Here, we addressed the problem of accurate structural validation with cryo-EM-based methodologies for determining the structures of up to megadalton-scale DNA objects in solution, together with molecular-dynamics-based methods for building pseudoatomic models in a semiautomated fashion. The library of objects includes four brick-like multilayer DNA origami objects with increasing internal floppiness, a barrel-like 126-helix bundle, two variants of a multidomain object called Twisttower, a design variant v2 of a previously reported object called the Pointer, a small 16-helix bundle, four variants of a hinged-beam-like object, two variants of a dumbbell-like object, and five variants of a six-helix tube featuring asymmetric markers at either end as reporters for twist and one ten-helix tube. We constructed pseudoatomic models for six different objects. The fitting was validated using Fourier shell correlation against the cryo-EM half-maps and the models show good cross-correlation with the cryo-EM maps.

The Twisttower design allowed us to systematically study twist deformations, and how they may be removed, in a square-lattice packing context as a function of cross-sectional area. To remove the global twist deformation, the internal design specifics must be changed such that the right-handed internal torques are mechanically balanced by counteracting left-handed torques. This may be achieved by locally deviating from the default eight-base-pair crossover spacing design rules following previously discussed concepts, by reducing the average bases between crossovers to achieve the native 10.5 base pairs per turn. We thus designed and solved a cryo-EM structure of a refined variant of the Twisttower in which we eliminated the global twist deformations. As a result, we obtained a more orderly object with a more regular square-lattice structure (right). We applied this analysis also to the twist-corrected variant of the Twisttower and the hinged-beam-like object v4.

> AAAAGAAGCCACCCTCCCGTCACCGACTTGAG;> TCATAAATCAGTTCAGAAAACGAGTCTAGCTGTGCCTGAGTACAAAAT;> ATTCATTGAATCCCCAAGAATAACTTAATTAAATAAGGAGAAACCA;> CATTACCGAGGGGGTAATAGTACACTATCA;> AAAATCAGAAATCACCTCAAATCACCATCAATGTCTGGAGTTTTT;> TTTTTTAAATTTAAAGAAGATGATGATTTTTTAACAAACATCAAG;> AGCCAGCATGAGGGAGGATAAAAATTTTTAGATAATCGTACAAACAAG;> TTCTGACCAATATATTTTAATGGAAACAGTTTTTTTACATAAATCAAT;> CCAGAGCCGCCATCTTGGCATTTTCGGTCTTTTTTTTTTATAGCCCCCTTATCCATCGAT;> TTAGTTAAAAGACAAACCGCGCCCAATAGCATCGTAGG;> TGATAGACGGTTTTTCGCCCTTTGACGTTGGAGTCCACGTTCTTTAATAGTGGACTCTTGTTCCAAACTGGAACAACACTCAACCCTATCTCGGGCTATTCTTTTGATTTATAAGGGATTTTGCCGATTTCGGAACCACCATCAAACAGGATTTTCGCCTGCTGGGGCAAACCAGCGTGGACCGCTTGCTGCAACTCTCTCAGGGCCAGGCGGTGAAGGGCAATCAGCTGTTGCCCGTCTCACTGGTGAAAAGAAAAACCACCCTGGCGCCCAATACGCAAACCGCCTCTCCCCGCGCGTTGGCCGATTCATTAATGCAGCTGGCACGACAGGTTTCCCGACTGGAAAGCGGGCAGTGAGCGCAACGCAATTAATGTGAGTTAGCTCACTCATTAGGCACCCCAGGCTTTACACTTTATGCTTCCGGCTCGTATGTTGTGTGGAATTGTGAGCGGATAACAATTTCACACAGGAAACAGCTATGACCATGATTACGAATTCGAGCTCGGTACCCGGGGATCCTCAACTGTGAGGAGGCTCACGGACGCGAAGAACAGGCACGCGTGCTGGCAGAAACCCCCGGTATGACCGTGAAAACGGCCCGCCGCATTCTGGCCGCAGCACCACAGAGTGCACAGGCGCGCAGTGACACTGCGCTGGATCGTCTGATGCAGGGGGCACCGGCACCGCTGGCTGCAGGTAACCCGGCATCTGATGCCGTTAACGATTTGCTGAACACACCAGTGTAAGGGATGTTTATGACGAGCAAAGAAACCTTTACCCATTACCAGCCGCAGGGCAACAGTGACCCGGCTCATACCGCAACCGCGCCCGGCGGATTGAGTGCGAAAGCGCCTGCAATGACCCCGCTGATGCTGGACACCTCCAGCCGTAAGCTGGTTGCGTGGGATGGCACCACCGACGGTGCTGCCGTTGGCATTCTTGCGGTTGCTGCTGACCAGACCAGCACCACGCTGACGTTCTACAAGTCCGGCACGTTCCGTTATGAGGATGTGCTCTGGCCGGAGGCTGCCAGCGACGAGACGAAAAAACGGACCGCGTTTGCCGGAACGGCAATCAGCATCGTTTAACTTTACCCTTCATCACTAAAGGCCGCCTGTGCGGCTTTTTTTACGGGATTTTTTTATGTCGATGTACACAACCGCCCAACTGCTGGCGGCAAATGAGCAGAAATTTAAGTTTGATCCGCTGTTTCTGCGTCTCTTTTTCCGTGAGAGCTATCCCTTCACCACGGAGAAAGTCTATCTCTCACAAATTCCGGGACTGGTAAACATGGCGCTGTACGTTTCGCCGATTGTTTCCGGTGAGGTTATCCGTTCCCGTGGCGGCTCCACCTCTGAAAGCTTGGCACTGGCCGTCGTTTTACAACGTCGTGACTGGGAAAACCCTGGCGTTACCCAACTTAATCGCCTTGCAGCACATCCCCCTTTCGCCAGCTGGCGTAATAGCGAAGAGGCCCGCACCGATCGCCCTTCCCAACAGTTGCGCAGCCTGAATGGCGAATGGCGCTTTGCCTGGTTTCCGGCACCAGAAGCGGTGCCGGAAAGCTGGCTGGAGTGCGATCTTCCTGAGGCCGATACTGTCGTCGTCCCCTCAAACTGGCAGATGCACGGTTACGATGCGCCCATCTACACCAACGTGACCTATCCCATTACGGTCAATCCGCCGTTTGTTCCCACGGAGAATCCGACGGGTTGTTACTCGCTCACATTTAATGTTGATGAAAGCTGGCTACAGGAAGGCCAGACGCGAATTATTTTTGATGGCGTTCCTATTGGTTAAAAAATGAGCTGATTTAACAAAAATTTAATGCGAATTTTAACAAAATATTAACGTTTACAATTTAAATATTTGCTTATACAATCTTCCTGTTTTTGGGGCTTTTCTGATTATCAACCGGGGTACATATGATTGACATGCTAGTTTTACGATTACCGTTCATCGATTCTCTTGTTTGCTCCAGACTCTCAGGCAATGACCTGATAGCCTTTGTAGATCTCTCAAAAATAGCTACCCTCTCCGGCATTAATTTATCAGCTAGAACGGTTGAATATCATATTGATGGTGATTTGACTGTCTCCGGCCTTTCTCACCCTTTTGAATCTTTACCTACACATTACTCAGGCATTGCATTTAAAATATATGAGGGTTCTAAAAATTTTTATCCTTGCGTTGAAATAAAGGCTTCTCCCGCAAAAGTATTACAGGGTCATAATGTTTTTGGTACAACCGATTTAGCTTTATGCTCTGAGGCTTTATTGCTTAATTTTGCTAATTCTTTGCCTTGCCTGTATGATTTATTGGATGTTAATGCTACTACTATTAGTAGAATTGATGCCACCTTTTCAGCTCGCGCCCCAAATGAAAATATAGCTAAACAGGTTATTGACCATTTGCGAAATGTATCTAATGGTCAAACTAAATCTACTCGTTCGCAGAATTGGGAATCAACTGTTATATGGAATGAAACTTCCAGACACCGTACTTTAGTTGCATATTTAAAACATGTTGAGCTACAGCATTATATTCAGCAATTAAGCTCTAAGCCATCCGCAAAAATGACCTCTTATCAAAAGGAGCAATTAAAGGTACTCTCTAATCCTGACCTGTTGGAGTTTGCTTCCGGTCTGGTTCGCTTTGAAGCTCGAATTAAAACGCGATATTTGAAGTCTTTCGGGCTTCCTCTTAATCTTTTTGATGCAATCCGCTTTGCTTCTGACTATAATAGTCAGGGTAAAGACCTGATTTTTGATTTATGGTCATTCTCGTTTTCTGAACTGTTTAAAGCATTTGAGGGGGATTCAATGAATATTTATGACGATTCCGCAGTATTGGACGCTATCCAGTCTAAACATTTTACTATTACCCCCTCTGGCAAAACTTCTTTTGCAAAAGCCTCTCGCTATTTTGGTTTTTATCGTCGTCTGGTAAACGAGGGTTATGATAGTGTTGCTCTTACTATGCCTCGTAATTCCTTTTGGCGTTATGTATCTGCATTAGTTGAATGTGGTATTCCTAAATCTCAACTGATGAATCTTTCTACCTGTAATAATGTTGTTCCGTTAGTTCGTTTTATTAACGTAGATTTTTCTTCCCAACGTCCTGACTGGTATAATGAGCCAGTTCTTAAAATCGCATAAGGTAATTCACAATGATTAAAGTTGAAATTAAACCATCTCAAGCCCAATTTACTACTCGTTCTGGTGTTTCTCGTCAGGGCAAGCCTTATTCACTGAATGAGCAGCTTTGTTACGTTGATTTGGGTAATGAATATCCGGTTCTTGTCAAGATTACTCTTGATGAAGGTCAGCCAGCCTATGCGCCTGGTCTGTACACCGTTCATCTGTCCTCTTTCAAAGTTGGTCAGTTCGGTTCCCTTATGATTGACCGTCTGCGCCTCGTTCCGGCTAAGTAACATGGAGCAGGTCGCGGATTTCGACACAATTTATCAGGCGATGATACAAATCTCCGTTGTACTTTGTTTCGCGCTTGGTATAATCGCTGGGGGTCAAAGATGAGTGTTTTAGTGTATTCTTTTGCCTCTTTCGTTTTAGGTTGGTGCCTTCGTAGTGGCATTACGTATTTTACCCGTTTAATGGAAACTTCCTCATGAAAAAGTCTTTAGTCCTCAAAGCCTCTGTAGCCGTTGCTACCCTCGTTCCGATGCTGTCTTTCGCTGCTGAGGGTGACGATCCCGCAAAAGCGGCCTTTAACTCCCTGCAAGCCTCAGCGACCGAATATATCGGTTATGCGTGGGCGATGGTTGTTGTCATTGTCGGCGCAACTATCGGTATCAAGCTGTTTAAGAAATTCACCTCGAAAGCAAGCTGATAAACCGATACAATTAAAGGCTCCTTTTGGAGCCTTTTTTTTGGAGATTTTCAACGTGAAAAAATTATTATTCGCAATTCCTTTAGTTGTTCCTTTCTATTCTCACTCCGCTGAAACTGTTGAAAGTTGTTTAGCAAAATCCCATACAGAAAATTCATTTACTAACGTCTGGAAAGACGACAAAACTTTAGATCGTTACGCTAACTATGAGGGCTGTCTGTGGAATGCTACAGGCGTTGTAGTTTGTACTGGTGACGAAACTCAGTGTTACGGTACATGGGTTCCTATTGGGCTTGCTATCCCTGAAAATGAGGGTGGTGGCTCTGAGGGTGGCGGTTCTGAGGGTGGCGGTTCTGAGGGTGGCGGTACTAAACCTCCTGAGTACGGTGATACACCTATTCCGGGCTATACTTATATCAACCCTCTCGACGGCACTTATCCGCCTGGTACTGAGCAAAACCCCGCTAATCCTAATCCTTCTCTTGAGGAGTCTCAGCCTCTTAATACTTTCATGTTTCAGAATAATAGGTTCCGAAATAGGCAGGGGGCATTAACTGTTTATACGGGCACTGTTACTCAAGGCACTGACCCCGTTAAAACTTATTACCAGTACACTCCTGTATCATCAAAAGCCATGTATGACGCTTACTGGAACGGTAAATTCAGAGACTGCGCTTTCCATTCTGGCTTTAATGAGGATTTATTTGTTTGTGAATATCAAGGCCAATCGTCTGACCTGCCTCAACCTCCTGTCAATGCTGGCGGCGGCTCTGGTGGTGGTTCTGGTGGCGGCTCTGAGGGTGGTGGCTCTGAGGGTGGCGGTTCTGAGGGTGGCGGCTCTGAGGGAGGCGGTTCCGGTGGTGGCTCTGGTTCCGGTGATTTTGATTATGAAAAGATGGCAAACGCTAATAAGGGGGCTATGACCGAAAATGCCGATGAAAACGCGCTACAGTCTGACGCTAAAGGCAAACTTGATTCTGTCGCTACTGATTACGGTGCTGCTATCGATGGTTTCATTGGTGACGTTTCCGGCCTTGCTAATGGTAATGGTGCTACTGGTGATTTTGCTGGCTCTAATTCCCAAATGGCTCAAGTCGGTGACGGTGATAATTCACCTTTAATGAATAATTTCCGTCAATATTTACCTTCCCTCCCTCAATCGGTTGAATGTCGCCCTTTTGTCTTTGGCGCTGGTAAACCATATGAATTTTCTATTGATTGTGACAAAATAAACTTATTCCGTGGTGTCTTTGCGTTTCTTTTATATGTTGCCACCTTTATGTATGTATTTTCTACGTTTGCTAACATACTGCGTAATAAGGAGTCTTAATCATGCCAGTTCTTTTGGGTATTCCGTTATTATTGCGTTTCCTCGGTTTCCTTCTGGTAACTTTGTTCGGCTATCTGCTTACTTTTCTTAAAAAGGGCTTCGGTAAGATAGCTATTGCTATTTCATTGTTTCTTGCTCTTATTATTGGGCTTAACTCAATTCTTGTGGGTTATCTCTCTGATATTAGCGCTCAATTACCCTCTGACTTTGTTCAGGGTGTTCAGTTAATTCTCCCGTCTAATGCGCTTCCCTGTTTTTATGTTATTCTCTCTGTAAAGGCTGCTATTTTCATTTTTGACGTTAAACAAAAAATCGTTTCTTATTTGGATTGGGATAAATAATATGGCTGTTTATTTTGTAACTGGCAAATTAGGCTCTGGAAAGACGCTCGTTAGCGTTGGTAAGATTCAGGATAAAATTGTAGCTGGGTGCAAAATAGCAACTAATCTTGATTTAAGGCTTCAAAACCTCCCGCAAGTCGGGAGGTTCGCTAAAACGCCTCGCGTTCTTAGAATACCGGATAAGCCTTCTATATCTGATTTGCTTGCTATTGGGCGCGGTAATGATTCCTACGATGAAAATAAAAACGGCTTGCTTGTTCTCGATGAGTGCGGTACTTGGTTTAATACCCGTTCTTGGAATGATAAGGAAAGACAGCCGATTATTGATTGGTTTCTACATGCTCGTAAATTAGGATGGGATATTATTTTTCTTGTTCAGGACTTATCTATTGTTGATAAACAGGCGCGTTCTGCATTAGCTGAACATGTTGTTTATTGTCGTCGTCTGGACAGAATTACTTTACCTTTTGTCGGTACTTTATATTCTCTTATTACTGGCTCGAAAATGCCTCTGCCTAAATTACATGTTGGCGTTGTTAAATATGGCGATTCTCAATTAAGCCCTACTGTTGAGCGTTGGCTTTATACTGGTAAGAATTTGTATAACGCATATGATACTAAACAGGCTTTTTCTAGTAATTATGATTCCGGTGTTTATTCTTATTTAACGCCTTATTTATCACACGGTCGGTATTTCAAACCATTAAATTTAGGTCAGAAGATGAAATTAACTAAAATATATTTGAAAAAGTTTTCTCGCGTTCTTTGTCTTGCGATTGGATTTGCATCAGCATTTACATATAGTTATATAACCCAACCTAAGCCGGAGGTTAAAAAGGTAGTCTCTCAGACCTATGATTTTGATAAATTCACTATTGACTCTTCTCAGCGTCTTAATCTAAGCTATCGCTATGTTTTCAAGGATTCTAAGGGAAAATTAATTAATAGCGACGATTTACAGAAGCAAGGTTATTCACTCACATATATTGATTTATGTACTGTTTCCATTAAAAAAGGTAATTCAAATGAAATTGTTAAATGTAATTAATTTTGTTTTCTTGATGTTTGTTTCATCATCTTCTTTTGCTCAGGTAATTGAAATGAATAATTCGCCTCTGCGCGATTTTGTAACTTGGTATTCAAAGCAATCAGGCGAATCCGTTATTGTTTCTCCCGATGTAAAAGGTACTGTTACTGTATATTCATCTGACGTTAAACCTGAAAATCTACGCAATTTCTTTATTTCTGTTTTACGTGCAAATAATTTTGATATGGTAGGTTCTAACCCTTCCATTATTCAGAAGTATAATCCAAACAATCAGGATTATATTGATGAATTGCCATCATCTGATAATCAGGAATATGATGATAATTCCGCTCCTTCTGGTGGTTTCTTTGTTCCGCAAAATGATAATGTTACTCAAACTTTTAAAATTAATAACGTTCGGGCAAAGGATTTAATACGAGTTGTCGAATTGTTTGTAAAGTCTAATACTTCTAAATCCTCAAATGTATTATCTATTGACGGCTCTAATCTATTAGTTGTTAGTGCTCCTAAAGATATTTTAGATAACCTTCCTCAATTCCTTTCAACTGTTGATTTGCCAACTGACCAGATATTGATTGAGGGTTTGATATTTGAGGTTCAGCAAGGTGATGCTTTAGATTTTTCATTTGCTGCTGGCTCTCAGCGTGGCACTGTTGCAGGCGGTGTTAATACTGACCGCCTCACCTCTGTTTTATCTTCTGCTGGTGGTTCGTTCGGTATTTTTAATGGCGATGTTTTAGGGCTATCAGTTCGCGCATTAAAGACTAATAGCCATTCAAAAATATTGTCTGTGCCACGTATTCTTACGCTTTCAGGTCAGAAGGGTTCTATCTCTGTTGGCCAGAATGTCCCTTTTATTACTGGTCGTGTGACTGGTGAATCTGCCAATGTAAATAATCCATTTCAGACGATTGAGCGTCAAAATGTAGGTATTTCCATGAGCGTTTTTCCTGTTGCAATGGCTGGCGGTAATATTGTTCTGGATATTACCAGCAAGGCCGATAGTTTGAGTTCTTCTACTCAGGCAAGTGATGTTATTACTAATCAAAGAAGTATTGCTACAACGGTTAATTTGCGTGATGGACAGACTCTTTTACTCGGTGGCCTCACTGATTATAAAAACACTTCTCAGGATTCTGGCGTACCGTTCCTGTCTAAAATCCCTTTAATCGGCCTCCTGTTTAGCTCCCGCTCTGATTCTAACGAGGAAAGCACGTTATACGTGCTCGTCAAAGCAACCATAGTACGCGCCCTGTAGCGGCGCATTAAGCGCGGCGGGTGTGGTGGTTACGCGCAGCGTGACCGCTACACTTGCCAGCGCCCTAGCGCCCGCTCCTTTCGCTTTCTTCCCTTCCTTTCTCGCCACGTTCGCCGGCTTTCCCCGTCAAGCTCTAAATCGGGGGCTCCCTTTAGGGTTCCGATTTAGTGCTTTACGGCACCTCGACCCCAAAAAACTTGATTTGGGTGATGGTTCACGTAGTGGGCCATCGCCC;> AACGGAGATTTGTATTAGGAATACAAAAGGATCAGGACGATGCCACT;> TTTTTGCGCGAAACACTAAAACCAGCGATAAGAGGCAGAGGACTAAAGACTTT;> TTGAGATTTTGTGAATTATACCAGAACGTAACCAGCATCGGAACGAGG;> CTGACCTTCATCGCCTCCATGTTAATTACGAGCGTTTACCAGACGACG;> GTAATCTTGACAAGATTGAAAGACTCCAAAACTAAAGGATTTTCACGGCTGAGGC;> TTTTGTTTTGTCCAGACAGCCCTCATTTTTTTTTTTAGTTAGCGTAAC;> AGACGTTAGTAAATGAATTGTATTCTTAAAC;> CGGTTTATCAGCTTGTTGAAAATTTTTT;> GTTTCAGCAGCTTGATCATCGCCCACGCATAAGCATGATTAACAGTTA;> GGAGTGAGTTGCGGGATCGTCACCCCCGTATA;> GTGAATAAGGCTTTTTTTTTTTTGCCCTGACGAGAAAACCCATGTCAGGGAT;> TCATTCATGGTTTAATTTCAACTTTAATCAAATTTTCT;> AAAGCTGCTTCAACAGTATGGGATTTTGCTGATCTAAAGCTTGAGA;> ACCGGATAGGAACAAAAAAGGCTCCAAAAGGAGCCTTTCATCAAGA;> GGTCAATCGACCAACTGAGGCTTTTTGCAGGGTTCGGAACCTATTATT;> TACGTTAATAAAATTTTTTTTTTCGAACTAACGGAACCTCATTTTTTT;> TTGGGAAGGGCTCATTACCTTATGCGATTTACACCAGATTACAGGT;> CAAAATAGCAGATACATAACGCCCACATTCAACTAATCAACATTATTTTT;> AAAAGCCTACCAGTATAAAGCCATATCATTCTGCAGAACGCTGAGAC;> TTACTAGACGGAATCGCCAACATGCAGAAGCAAAGCGGAT;> TTTTTCGTTAAATATGGTTTGAAATATTTTTTCCGACCGTGTGAT;> ACGAAGGCGTACCGACTTTTGCCAATTAGCAAGGCCGGAACCGTAATC;> AAAACGAAATCCGCGCGCAGACAGGCGCATAGGCTGG;> AAATTCTTGTTTAGTATCATATGAAAGAATAAAATGTTTAGCCAGTA;> CCATTAAATAGTACCGGTGCCGTCTTACCAGCGCCAAAGA;> TTCATGAGAACGAGGACCTGCTGATAAATTGTGTCGATATACCAATACAGACC;> GGTATTAAACCAAGTCGTTATACCATTTTCGAGACTGGA;> TCGGCTGTCTTTCCTACGCTCAATAACAACG;> CAGTACAACAATAGGTAAGAACTAAAAATCAGAAAGATTCATCAG;> CGCCTGTATTCGTCACAGTATAGCCCGGATTTTTTTTTTATAGGTGTATCAC;> GCCGCTTAATAGAAATTCATTACCCAAATCCTTAGCCGGGAAGTTT;> AGTTAAAGTTCGGTCCTTTCGAGGTGAATT;> CCAGCTACAGCGTCTTTCCAGAGTAGACGGGGAACAAAG;> TTTTGCATTCCAGGTAATAAGTTTTTTTTTTTTTTAACGGGGTCAGTG;> AAGACTCCAATACATACATAAAGGTGGAAAGCATAAATCC;> GAGGAAACGCTAACGAATTTTATCCTGAATACCGCACT;> TATCCCAACAGATATAGAGTACCTTTAATTGCTGTACCAACATTAACAGAACCTAC;> TATTATTGCCAGTTACAAGATTAGTTGCTATTATTTTC;> AACAGTGCTCAGCAGCAACAACACCGATAGTTGCGCCGTCTTTCC;> GAAGGCTTATCCGGTCCTTAAATCAAAATAGAACCTCCGAGAGAAT;> ATTCTAAGAACGCTTTTTTGAGGCGTTTTAGCATATAACTTAACCTCC;> GCGGATAAAAAAGGTAACGGAAATTATTCATT;> TTAGGATTCAATAAACGTTTTAATGTCTTTACGATTCAAAAGGGTGAG;> AAGCAAATGCGCCTGTAAGAGGAAGCCCGAAAAAATGCAAAAACATTA;> CAGCTAACAAGAACGACAAGCAAGCCGTTTTTTTGCACATTAAGAGTTACCAGA;> TTATCAACAATAGATATCAATAAAATCATTCCATCCTATTTTGAAG;> AAGTCCTGAACAATTTTTTGAAAAATAATATCAGAACGCGATGCAAAT;> AGAACCGCCACCCTTTTTTTTTTTCAGAGCCACCACTAGCGTTTTTTT;> ATATAAAACCAACCTTAACCCTGCATAGTAAGAGCAACAAAGTAC;> ATAAGAGACTGTCCAGACGACGAAGCGGGGT;> CCATATTCAGTAGGGACACCGGAATCATAA;> CAGGAAGAACAATAATTTGAATTACCTTTT;> ATGAATATTAGATTTTGTTATTAATTTTATTTTTTTTTTAAAGTTTGAGTAA;> GTAAACGTAGGGTTATCCAATAAATCATAC;> CCAATAGGTGTTAAATTCGGCCTCACCGCTTCCAGCAACCGCAAGAATTGGGTAAA;> ACTTCTGACATCTGCCCCGTCGGAAAGGGAAGAAAGCGAAAGCGGTCA;> TGGATTATCATATCAAAATTATTTTTGTATA;> GATTGTTGAGTCAATAGTGAATGGCTTAGGGACCATTGTTAAGCC;> TTTTTAACGCCATAACGGCGGATTGACCGCGGGGAAA;> AACTGTTGGGAAGTTTTTTTTTTGGCGATCGGTGCGTCGTCTCGTCCGGCAA;> GGCCTCTTCGCTATTCTTTGAATGATAATCTGACCCTG;> CAACCGATAAGACACCATAAAGCCTCAGAGCATTGTTAAACATATGTA;> CGGAAGCAAACTCCAACAGGTCAGAAAGATT;> GATACAGGGGAGGTTGCCTCAGAGCCGCCTTTTTTTTTTACCAGAACCACCAACCGGAAC;> GAAAATTCCGTAGAATTATTACGCAGTATGGACAATGAACTACAAAAACAACT;> TTTGTCACAATCAATAACAAACAAGCAGTCTC;> ACGGAATATATAAAATACCCAAAAGAACTGCCGATATA;> GTCATTTTTCGAGCTTTTTGCGGGAGAAGCCTTTATTTCATTAAGCA;> TTTTTAGTGTACTAGTAAGCGTCATATTTTTTTTTTCATGGCTTTTGATTTGGCCTT;> TGGCAACAAGTTTATATGCCCCCGTACCAGGTAGCAACGGCTACA;> GCTTAGAGCTTAATTAGGAAACCGATAGCCAGAATTAATGAGCGC;> GCTGAATACAACTAAAAGTAGTAGTAACCTGTTCTGGCCTTCCTGTAG;> TGAATTTACCGTTCCTTAGCAAACAGACGACCTTGAGTTGATATA;> ATTAAGACTCTGTAAAAGCAAATATTTAAATTGGCAAAGCAGTTTGAG;> ATAGCGATAGCTTAGTAGCTCAAGATTAGA;> TCATTAAAGCCGCCACAAAAGGGCGACATTTTTGCTCATGCCTAT;> TAAAGCTATAATACTCAAAGCGAACCAGACTCCTCAAGTGAAAGT;> AATCGGTTCCTTTTGATAAGAGCTGAAACAAGAAGGACATCGAGA;> TCGTCGCTATTAATTCCAATCGCTTGGGTTAACAGCCA;> AATTTTCCCTTAGTTTTTTAATCCTTGAAAACAAACAGAATCATCAAT;> CCACCACAGGCAGGTCAAAATCCGTACTCAGGAGGTTCGGGTAAACGAAAGA;> CCCTCAGAAACCGCCTCCCTCAGAAGTTTGCCCATTTGG;> ACCTTGCTCAATTTCACGGATTCGCCTGATTG;> ACCACCGGACCGCCACCCTCAGAGGATATTC;> ACCCTCATAGGTAAACCTGACTATAAATCATAGCGTCCAATACTG;> TTTCATCTTCATAATAATGAAAGCGAGAGGCTTTTGCATAAAAACATACGTA;> TCAGACTGTAGCGCGTCAGAGCCAAAGGTGAATATGGTGAGAGGGT;> CTTTAGCGAGTAGCGACAGAATCAGAGACAGAGTAGCACGAATTAG;> AAAGGCCGACGCAAGGGAAGGTAAATATTGAAGTAATT;> TAATGTGTATATTTTGACTTCAAATATCGCAACATGTTGCAGAGG;> ACATTTAAATAAATTATCTACAAAGGCTATCATAAAACGATGGCGAAA;> AGCAGCAACGTCACCATTATCAAGAACCGCCACCCTCAGCAAGCC;> ATGATATTCAACCGTAATGACCATTATAGTTAATTTAG;> ATGCCGGAGAGGGTACTCAAATGTTTCATCGAGAATCG;> CCCTGAACCTTACCAACGCAATAATAACGGAAGAAACGCA;> TTTTTAAAGTCAGATCTTACCGAAGCTTTTTTTTTTCCTTTTTAAGAAA;> TAATATCAGAGAGATAAAGAGCAATCCAAATATAAATATGTAATGCTG;> GAAATAGCAATAGCTAGGGTAATCTGAACA;> GAAACAATTCTGCGAACGAGTAGAATGGTCAAGCTGAGAA;> CAATAATACCCACAAAACAGGGAAGCGCATCCTAATTT;> AGAAACGATTTTTTGAACATAAAGAATTGACCTTTACATTTTT;> TTTAACGTCAAAATTTTTTATGAAAATAGCAGTACCTTTTTTTTT;> GTTTCATTTGCGGATGAGGCAAGGCAAAGAATTAGCAAAAGCCAGAA;> TTTTCCATATAATTTGGGGCGCGAGTTTTTTTTTTCTGAAAAGGTGGC;> TTAGCTATATTTTCACAGTTGATTCTGGAAAGTAAGCA;> AGATACATTTCGCAATTTAGTTTCATGTTT;> TTATCAAAATCATTTTTTTAGGTCTGAGAGACATGGCAATTTTTT;> TTTTTCTGAGCAAGAATTGAGGAAGGTTTTTTTTTTTTATCTAAAATAT;> CGCGCAGACAACTAATCGGCCAGTGAACGGATAACCTCAC;> ATTCATTAAAACAAAATTAATTTGCATCAACTTTAAA;> TCAATTACTTTTACATTACATTTGAGGATTTTTTTTTTTTTAGAAGTATTAG;> CGGGAGAAACGTCAGATATGTGAGTGAATA;> AGAAAAGCCCCAAAAACGACAACTAGATTAGATTTTGAAT;> CCTTCTGACTTGCTGGATTAGTAATAACATTTTTTTTTTTCACTTGCCTGAGTTTTTATA;> ACTTTCTCCGGCCTTTAGTGATGAAGGGTAAACTTAAATGAGACGCA;> AATTTGTGAGAGATAGCGGAAAAATTCTGCTC;> ATCGGCGCCAGTCACGACGTTGGGTCATTGACCAAGT;> TTTTTGTTGAAAGCTCAATCAATATCTTTTTTTTTTTGGTCAGTTGGCATACCGAAC;> TTTTTAAAAAAGCTTGGGCGGATAAAAAAAAGGGATAGCTCTCA;> ACTGATAGGGCTATTAATTCACCAGGAAAAACGCTCATGGCCATCAC;> CCCTAAAACAGCAGAATGCTGAACCTCAAATATCAAACCGTGGAGCC;> CATCGCCAGCCACGGGCCAAGCTTTCAGAGGCTATTTT;> TTAAAAACTTTAGGAGCACTAAGGCGAATTTGAGAGA;> ACGCCAGCGCCATTCGCACATCCTCATAACGG;> AGGCGATTGGGTTTTCAAACGTACAGCGCCAT;> GGGGGATGTGCTGCAAGAATCGACCTGAGA;> CAACAGCTCGTGCCAGCTGCTTTTTTTTTTATTAATGAATCGGCCAGTCGGTTCACGGT;> GGGAACACAAAAATATTTTTAAATCAATTCTACTAATGTACGGTGTCCCAAT;> GTAACAACAAACCACCTAAACAGGAGGCCGATGCCGCGCT;> GGGCGCCAGGATCCCCGGGTACCGCCTCCTC;> TAGATGGGGCCTGGGGTGCCTAATAAGCACTAGAGCTTGAGGGTCGAGTTTTT;> CGCATCGTAACCGTGATAATGGAATTCGCG;> ATCATCATATTCCTTTTTTTTTTTGATTATCAGATGGTGCTTTCTTTTT;> TCATGGTCATACCGGGGGTTTTTTTTTTTTTCTGCCAGCACGCGGGCCGTTTTTTT;> ATTCGTAACGGGGAGAGGCGGTTTCACCAGT;> AGGAAGATCAACATACGAGCCGGATCCCTTAC;> GAACAAAGCGTATTAATAGAACGTCAGCGTGGGCAAATTA;> ATCCTTTGCCCGAACCAGGTTTAGCACGTA;> CAGCTTAGTGCCTGTTCTTCGCGTCCGTGAGAGCTCGATGTGAAATGCGTTGCG;> GTCGGTGGTGCCATCCAGCATCAGCAGATGCCCCCTGCATTAAATCAA;> TGCTGGTCTTTTAGAGGGACGACGACAGTACAGCTCATTAATATT;> TGTTATCCAACGGCATCGGGGTCAGCGCGGTTCAGACGATCCAGCGCA;> GCTCACAACAGCACCACAGTTGAAGCCAGCTTTCCGGC;> AGCATAAATGGTCAGTGGTGCCGGAAACCA;> CAGGAACGGTACGCCAAGGCCACCACCGTTGT;> TAGAAGAACTCGTTAGACTATGGTCGTATAACGGCGCTGGCAAGTGT;> TTTTGAAACCTGTCCAGTTTGGAACTTTTTTTTTTAAGAGTCCACTAT;> GCCTGGCCCTGAGAGACCAGCAGGAAAGGGCGACGTGAACGCGGTATG;> AAGCGGTTAATGGGAGGGTGGTTTTTCTTTTGCGTATTCATTAATT;> GCCGGCGACCGATTTAAATCGGAACCCTAAAGATAAACA;> AGGAGCGGCGGGAGCAGAAGGAGCGGAATTATAATCCTCATCAAC;> TGGTGGTTGATTGCCCTTCACCGAGACGGG;> CGCTGCGCGTAACCACGGAGCCCACGTGGCGGTGTAAA;> GTGGACTCTCACTGCCCGCTTTCCAACGCG;> CCAACGTCCGAAAATCATCCCTTACATCACCCAAATCAAG;> TAATGCGCCGCTACAGATCAGTGGAATCCTGGGACTTG;> GGCGCGTAATCAGAGGCGCTAGATTAAATGTGAGCGACCAGCTTT;> CTGTGGTGCTGCGTTTTTTTTTTGCCAGAATGCGGCTGCGCGCCTTTT;> ACTGGTGTGCCCTGCGGTGCCGTAGGGCGATGGCCCACTAAAAACCGAATCGTT;> GAGTAAAAGAGTCTGTCACACCCTAAAGGGAAGAAAGGTTCTCCGT;> GCTTTCGGCCAACGGTTCCACACGCACTCCTAGGTCACGTTGGTG;> GGTTTCTTTGCTCGTCAAATACCAGCCTCCGCGTTTTT;> AGCAATACCCAGCCAAACGTGCCACAATATGCCGTCAATAGATAA;> TTCTTTGTAATATCCAGAAGTGCATTATCATTTTGCG;> GTGTCACCGGCTGGAGGTGTCCCACGCAACTTTCCTG;> TTTTTGCTGGTAACACTCAATCCGCCGGTTGCAGGC;> AGCCGGGTCACTGTTGTTCAGCATCTATCAGAGTGAGC;> TAGGGTTGTGTGCACTAGCGGTGCCGGTGCCGGGTTACC;> AAGAATAGCCCGAGATAAAGAACTGCAGCCCATAGCTG;> TTTTTAGTGTTGTTCCGAAATCGGCAAACTGTTTGA;> TTTTTTGCCACGCTGGTTTGCCGTTGCAGCTAACTCA;> TTGCAACAGTCACACGACCAGTAAGAACCAC;> TAAAAGGTGGCACAGAGAACAAACTTTACAAACAATT;> GTCTTTAAGCCAGAGCCATTCAGGCTGCGCCCCCGGTTTGAACGG;> TTTTTTCGCTGGCTACATTTTAAATGGATTATTTACAGGCGGTCACGCGGTC;> AATCAACAAGAATACGGACATTCTGGCCATTTTTTTTTTACAGAGATAGAACTATTACCG;> ATTTGCCGCCAGCAGCGCACAGGCGTGGTGATCCCGTATTTTT;> AGTATTAAAGCAGCAAATGAAAAATCTAAAGCGGAAACATGCGCGA;> GAAACAGCGCCACGCGTTTACCAGATGCTGATTGCCGT;> TGAGAGCCCACCGCCTGCAACAGTGGATCAAAGTTAAACGTCCCGG;> CATCACCTGATAAAACAGAGGTGATTGGCAG> MRNEMHLQFSARSENESFARVTVAAFVAQLDPTMDELTEIKTVVSEAVTNAIIHGYNNDPNGIVSISVIIEDGVVHLTVRDEGVGIPDIEEARQPLFTTKPELERSGMGFTIMENFMDEVIVESEVNKGTTVYLKKHIVKS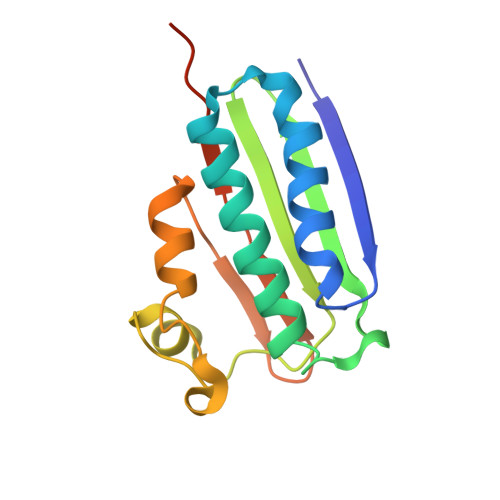KRYLEGSSF> VFPSNATFGMGDRVRKKSGAAWQGQIVGWYCTNLTPEGYAVESEAHPGSVHIYPVAALERIN

Plasmid-encoded bacterial R67 dihydrofolate reductase (DHFR) catalyzes the same reaction as the chromosomal counterpart but is highly resistant to the widely used antibiotic Trimethoprim (TMP) unlike the chromosomal enzyme. Dihydrofolate reductase (DHFR) catalyzes the reduction of dihydrofolate (DHF) to tetrahydrofolate (THF) employing nicotinamide adenine dinucleotide phosphate (NADPH) as a cofactor. Of special interest is R67 DHFR, a type II R-plasmid encoded DHFR that is distinct from the bacterial- and mammalian- chromosomal DHFRs in sequence, structure, catalytic, and inhibitory mechanisms. The active site of R67 DHFR is a promiscuous binding surface as evidenced by the binding of, NADPH and DHF for catalysis, a-NADH as an alternative cofactor, and novobiocin (Ki = 70 µM) and Congo red (Ki = 2 µM) as inhibitors that do not resemble either NADPH or folate.

The structure of Q67H mutant of R67 DHFR complexed with a non-specific inhibitor Congo red (CGR) has been determined at 1.15 Å resolution. R67 DHFR-CGR binary complex crystals belong to the space group I4122 as in previously determined structures. In the Fo-Fc map, one of the two naphthalene moieties in CGR is clearly observed, however, the biphenyl linker and the other naphthalene moiety are not seen owing to flexibility. CGR does not utilize its twofold axis to align with any of the three crystallographic twofold axes of the tetrameric protein instead, it binds like the asymmetrical folate and NADP+ at any one of the four symmetry-related positions in the active site pore. The naphthalene moiety with exocyclic sulphonate ion and amino group, interacts with residues 66–68 from all four protomers via metal-based ionic, van der Waals, stacking, and hydrogen bonding interactions. Amino acid residues Val66, His67, and Ile68, with their symmetry-related partners form the immediate vicinity of the bound sulphonated naphthalene. The exocyclic amino group of the naphthalene ring is involved in water-mediated interactions with subunit D. The aromatic naphthalene ring forms a C-H···O interaction with a water molecule that is H-bonded with the carbonyl oxygen of Val66 of subunit C. The naphthalene ring has stacking interactions with a pair of imidazole rings from symmetry related His67 residues. So, we conclude that CGR can bind in any of the four symmetry-related positions, however, only one CGR is bound at any given time due to stereochemical reasons leading to a stoichiometry of one CGR per tetramer. In striking contrast to bisbenzimidazole inhibitors, Congo red does not use its symmetry for binding and the sulphonate does not interact with Lys32 or YTT cluster. In our work, CGR is bound asymmetrically between two anti-parallel β strands in the active site pore with no changes in the protein structure.4-[4-(4-aminophenyl)buta-1,3-diyn-1-yl]-N-[(2S,3R)-3-hydroxy-1-(hydroxyamino)-1-oxobutan-2-yl]benzamide | C21 H19 N3 O4 | 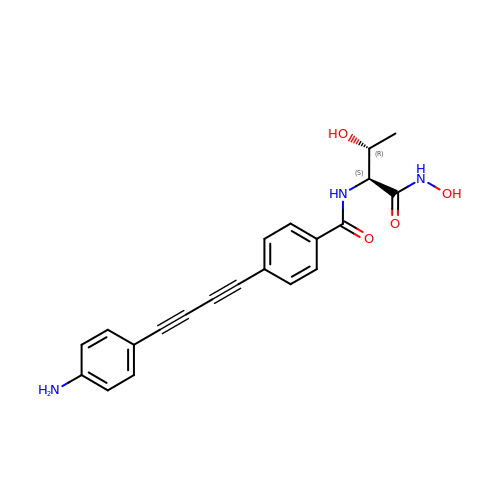SNVYDNOGPYZQEV-KUHUBIRLSA-N> MDLVKDVKRELSFSELKGKRVSIDGYNALYQFLAAIRQPDGTPLMDSQGRVTSHLSGLFYRTINILEEGVIPIYVFDGKPPEQKSEELERRRKAKEEAERKLERAKSEGKIEELRKYSQAILRLSNIMVEESKKLLRAMGIPIVQAPSEGEAEAAYLNKLGLSWAAASQDYDAILFGAKRLVRNLTITGKRKLPNKDVYVEIKPELIETEILLKKLGITREQLIDIGILIGTDYNPDGIRGIGPERALKIIKKYGKIEKAMEYGEISKKDINFNIDEIRGLFLNPQVVKPEEALDLNEPNGEDIINILVYEHNFSEERVKNGIERLTKAIKEAKGASRQTGLDRWF;> MMKAKVIDAVSFSYILRTVGDFLSEANFIVTKEGIRVSGIDPSRVVFLDIFLPSSYFEGFEVSQEKEIIGFKLEDVNDILKRVLKDDTLILSSNESKLTLTFDGEFTRSFEL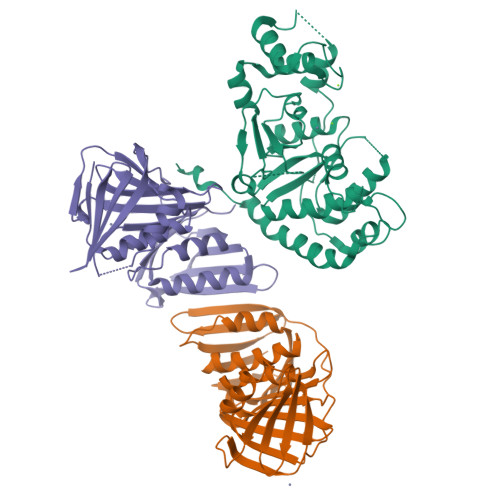PLIQVESTSPPSVNLEFPFKAQLLTITFADIIDELSDLGEVLNIHSKENKLYFEVIGDLSTAKVELSTDNGTLLEASGADVSSSYGMEYVANTTKMRRASDSMELYFGSQIPLKLRFKLPQEGYGDFYIAPRAD;> MFKIVYPNAKDFFSFINSITNVTDSIILNFTEDGIFSRHLTEDKVLMAIMRIPKDVLSEYSIDSPTSVKLDVSSVKKILSKASSKKATIELTETDSGLKIIIRDEKSGAKSTIYIKAEKGQVEQLTEPKVNLAVNFTTDESVLNVIAADVTLVGEEMRISTEEDKIKIEAGEEGKRYVAFLMKDKPLKELSIDTSASSSYSAEMFKDAVKGLRGFSAPTMVSFGENLPMKIDVEAVSGGHMIFWIAPRL> GSMTLSSNQYQLPLNVRPYTTTWCSQSPSCSNLLAIGHDTGITIYCASEEQTPGSTGLTLQELFTIQTGLPTLHLSFSSSCSYSENLHDGDGNVNSSPVYSLFLACVCQDNTVRLIITKNETIITQHVLGGKSGHHNFVNDIDIADVYSADNRLAEQVIASVGDDCTLIIWRLTDEGPILAGYPLSSPGISVQFRPSNPNQLIVGERNGNIRIFDWTLNLSAEENS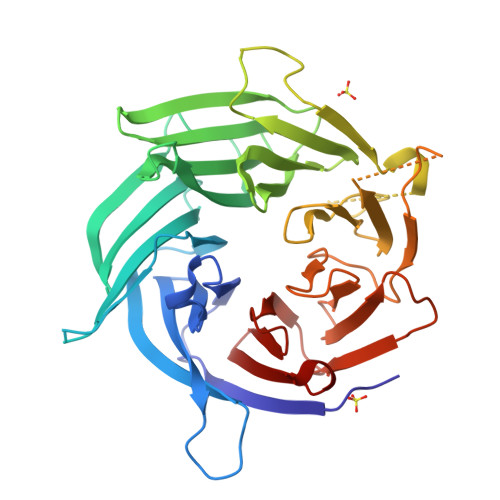QTELVKNPWLLTLNTLPLVNTCHSSGIASSLANVRWIGSDGSGILAMCKSGAWLRWNLFANNDYNEISDSTMKLGPKNLLPNVQGISLFPSLLGACPHPRYMDYFATAHSQHGLIQLINTYEKDSNSIPIQLGMPIVDFCWHQDGSHLAIATEGSVLLTRLMGFTRL> MSTLYEKLGGTTAVDLAVDKFYERVLQDDR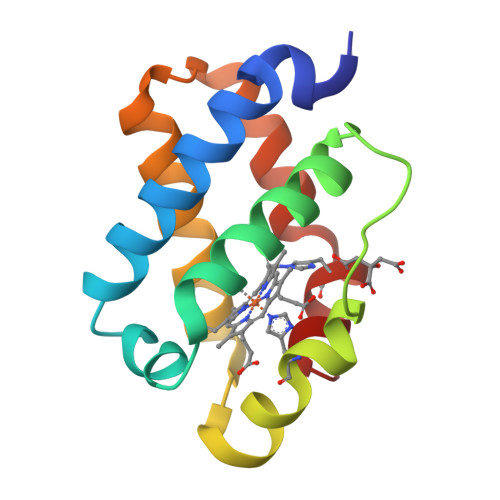IKHFFADVDMAKQRAHQKAFLTYAFGGTDKYDGRYMREAHKELVENHGLNGEHFDAVAEDLLATLKEMGVPEDLIAEVAAVAGAPAHKRDVLNQ> GSFPSTVKNGLSKIGIPSNVLDFMFDWTGSDQDYPKVPEAKGSIQAVRNEAFFIPLYELFLTYGGIFRLTFGPKSFLIVSDPSIAKHILKDNAKAYSKGILAEILDFVMGKGLIPADGEIWRRRRRAIVPALHQKYVAAMISLFGEASDRLCQKLDAAALKGEEVEMESLFSRLTLDIIGKAVFNYDFDSLTNDTGVIEAVYTVLREAEDRSVDPIPVWDIPILKDIVPRQRKVATSLKLINDTLDDLIATCKRMVEEEELQFHEEYMNERDPSILHFLLASGDDVSSKQLRDDLMTMLIAGHETSAAVLTWTFYLLTTEPSVVAKLQEEVDSVIGDRFPTIQDMKKLKYTTRVMNESLRLYPQPPVLIRRSIDNDILGEYPIKRGEDIFISVWNLHRSPLHWDDAE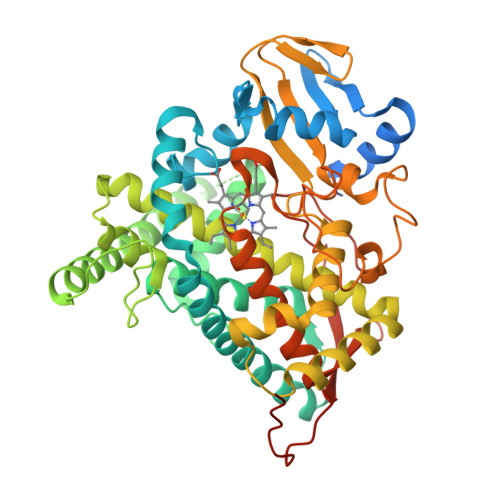KFNPERWPLDGPNPNETNQNFSYLPFGGGPRKCIGDMFASFENVVAIAMLIRRFNFQIAPGAPPVKMTTGATIHTTEGLKLTVTKRTKPLDIPSVPILPMDTSRDEVSSALS>GHMERLLDELTLEGVARYMQSERCRRVICLVGAGISTSAGIPDFRSPSTGLYDNLEKYHLPYPEAIFEISYFKKHPEPFFALAKELYPGQFKPTICHYFMRLLKDKGLLLRCYTQNIDTLERIAGLEQEDLVEAHGTFYTSHCVSASCRHEYPLSWMKEKIFSEVTPKCEDCQSLVKPDIVFFGESLPARFFSCMQSDFLKVDLLLVMGTSLQVQPFASLISKAPLSTPRLLINKEKAGQSDPFLGMIMGLGGGMDFDSKKAYRDVAWLGECDQGCLALAELLGWKKELEDLVRREHASIDAQS[2x]

Sirtuins constitute a family of NAD+-dependent enzymes that catalyse the cleavage of various acyl groups from the ∊-amino group of lysines. Sirtuins consist of a highly conserved catalytic deacylase domain of around 275 amino acids that is flanked by unstructured N- and C-termini that differ in their length and in their sequence. Of the seven members of the human sirtuin family, Sirt2 is mainly found in the cytoplasm, while Sirt3 is the main mitochondrial deacylase.

Using the diffraction data obtained from the soaked crystals, we were able to solve the crystal structures of Sirt2 in complex with ADPR and either EX243 (EX243 is the S-enantiomer of EX527; Sirt2–ADPR–EX243 structure) or CHIC35 (Sirt2–ADPR–CHIC35 structure) by molecular replacement. The asymmetric unit contains two monomers that show no significant differences [r.m.s.d.s of 0.29 Å (Sirt2–ADPR–EX243) and 0.23 Å (Sirt2–ADPR–CHIC35) for all Cα atoms]. The ADPR molecules of both structures assume a position that is almost identical to that observed in the Sirt2–ADPR complex. To our surprise, each Sirt2 molecule contained well defined electron density for two indole molecules. One indole mimics the physiological sirtuin inhibitor nicotinamide and occupies the C-pocket and the adjacent extended C-site. The other inhibitor molecule binds to the selectivity pocket of the hinge region. The carboxamide of both indole inhibitors binds in a similar fashion as the carboxamide moiety of the physiological inhibitor nicotinamide and hydrogen-bonds to the highly conserved residues Ile169 and Asp170 and, via one of the water molecules (W24 in Sirt2–ADPR–CHIC35 and W206 in Sirt2–ADPR–EX243), to Ala85, Ile93 and Pro94. The amide of the indole hydrogen-bonds to Gln167 and, via the other highly coordinated water (W3 in Sirt2–ADPR–CHIC35 and W203 in Sirt2–ADPR–EX243), to Asp168 and ADPR. The binding of the hinge molecule is mainly driven by hydrophobic inter­actions with the side chains of Ala135, Leu138, Tyr139, Phe143 and Phe190. The hinge molecule may supposedly be of no physiological relevance for Sirt2 inhibition, but it highlights the adaptability of the hinge region of Sirt2 and the selectivity pocket.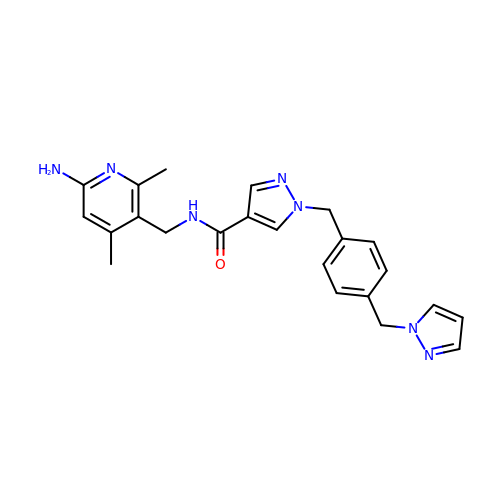N-[(6-amino-2,4-dimethylpyridin-3-yl)methyl]-1-({4-[(1H-pyrazol-1-yl)methyl]phenyl}methyl)-1H-pyrazole-4-carboxamide | C23 H25 N7 O | OINOKQVNBGAIMA-UHFFFAOYSA-N Sialin, a member of the solute carrier 17 (SLC17) transporter family, is unique in its ability to transport not only sialic acid using a pH-driven mechanism, but also transport mono and diacidic neurotransmitters, such as glutamate and N-acetylaspartylglutamate (NAAG), into synaptic vesicles via a membrane potential-driven mechanism. Sialin (SLC17A5) belongs to the solute carrier 17 (SLC17) transporter subfamily that includes nine related transmembrane major facility superfamily (MFS) transporters, all of which are dedicated to anion transport, including the vesicular glutamate transporters 1-3 (VGLUT1–3) and a vesicular nucleotide transporter (VNUT). Sialin adopts a classical MFS fold consisting of 12 transmembrane helices (TMs) with two pseudo-symmetric domains: N-domain (TMs 1-6) and C-domain (TMs 7-12). The Sialin structures in both the lumen-open and cytosol-open conformations reveal a solvent-accessible cavity, which forms the substrate translocation pathway, at the center of the interface between the N-domain and C-domain.

To capture the lumen-open state, we introduced a mutation on Arg168. This residue has a hydrophilic interaction with the carbonyl of Arg57, stabilizing TM1 which in turn presumably confines the conformation of TM7 in the cytosol-open state via a direct interaction between the hydroxyl group of Ser61 and the main chain carbonyl of Leu309. The cryo-EM structure of the SialinR168K complex with Fab10B8 in the apo state at pH 7.5 was determined at 3.3-Å resolution and exhibits a lumen-open conformation. Lys168 forms a salt bridge with Glu171 and does not bind to the main chain carbonyl of Arg57. Indeed, the S61A and R168K mutations confine Sialin in the lumen-open state, indicating the importance of these residues in regulating the conformation of Sialin. Dali search shows that the overall structure of SialinR168K shares a similar fold with, VGLUT2 and monocarboxylate transporter 124 (MCT1) with R.M.S.D. values of 1.2 Å and 2.4 Å. In the lumen-open state, the cytosolic end of TM8 shifts more than 12 Å towards the N-domain around the kink at Ser332 on the lumen leaflet, and the luminal end of TM7 and TM11 shifts by over 9-Å away from the N-domain. The lumen-open structure reveals that the hydrophilic interactions between Arg195 on TM5 and Gln273 on the cytosolic helix, Ser196 on TM5 and Arg353 on TM8, Lys197 on TM5 and Asp350 on TM8 seal the substrate translocation pathway from the cytosolic space. Therefore, we employed Glide28 to dock the sialic acid into the cavity. The top three positions are similar, suggesting that His298, Tyr301, and Ser411 form hydrophilic interactions with sialic acid.

> MDYKDDDDKRSPVRDLARNDGEESTDRTPLLPGAPRAEAAPVCCSARYNLAILAFFGFFIVYALRVNLSVALVDMVDSNTTLEDNRTSKACPEHSAPIKVHHNQTGKKYQWDAETQGWILGSFFYGYIITQIPGGYVASKIGGKMLLGFGILGTAVLTLFTPIAADLGVGPLIVLKALEGLGEGVTFPAMHAMWSSWAPPLERSKLLSISYAGAQLGTVISLPLSGIICYYMNWTYVFYFFGTIGIFWFLLWIWLVSDTPQKHKRISHYEKEYILSSLRNQLSSQKSVPWVPILKSLPLWAIVVAHFSYNWTFYTLLTLLPTYMKEILRFNVQENGFLSSLPYLGSWLCMILSGQAADNLRAKWNFSTLCVRRIFSLIGMIGPAVFLVAAGFIGCDYSLAVAFLTISTTLGGFCSSGFSINHLDIAPSYAGILLGITNTFATIPGMVGPVIAKSLTPDNTVGEWQTVFYIAAAINVFGAIFFTLFAKGEVQNWALNDHHGHRH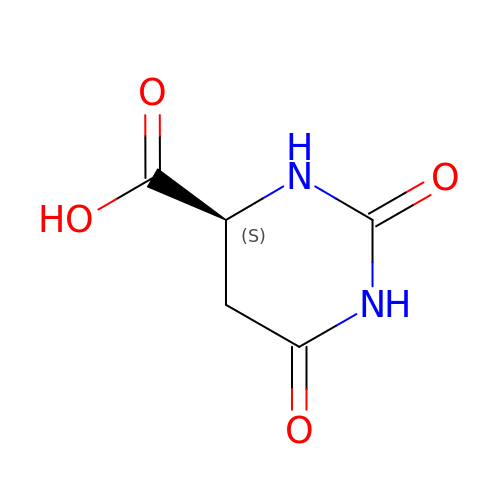(4S)-2,6-DIOXOHEXAHYDROPYRIMIDINE-4-CARBOXYLIC ACID | C5 H6 N2 O4 | UFIVEPVSAGBUSI-REOHCLBHSA-N(2R)-3-{[(S)-hydroxy{[(1R,2R,3R,4R,5S,6R)-2,3,5,6-tetrahydroxy-4-(phosphonooxy)cyclohexyl]oxy}phosphoryl]oxy}propane-1,2-diyl dioctanoate 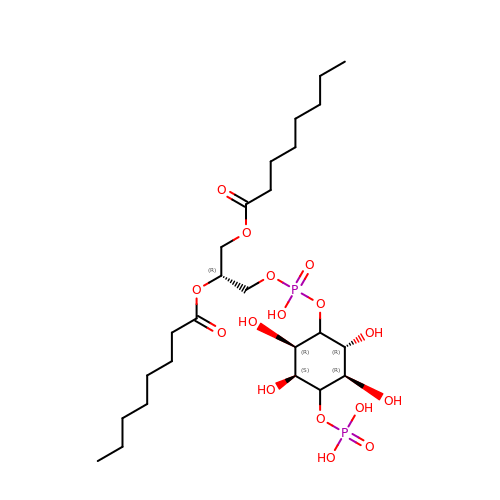| C25 H48 O16 P2 | SNIQYSSXZJPPEL-LKTRINTESA-N>[2x]FSMKIGIIGAMEEEVTLLRDKIENRQTISLGGCEIYTGQLNGTEVALLKSGIGKVAAALGATLLLEHCKPDVIINTGSAGGLAPTLKVG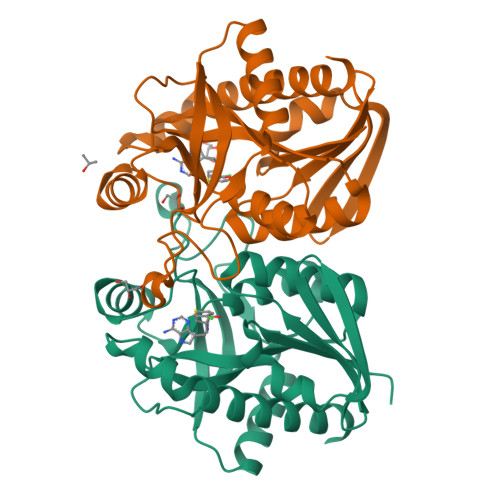DIVVSDEARYHDADVTAFGYEYGQLPGCPAGFKADDKLIAAAEACIAELNLNAVRGLIVSGDAFINGSVGLAKIRHNFPQAIAVEMEATAIAHVCHNFNVPFVVVRAISDVADQQSHLSFDEFLAVAAKQSSLMVESLVQKLAHG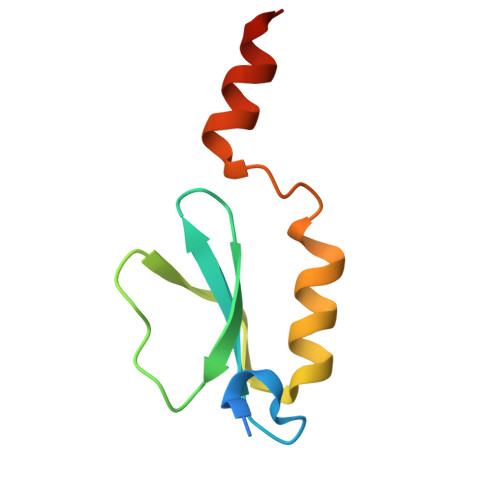> AMADIGSMTNPFDDDEGVFLVLVNDEDQYSLWPEFAEVPQGWRTVFGPTSRAAALDYINTHWTDLRPRSLREAMEAHSTAG> PIRLPNPMIGFGVPNEPGLITHRSLPELARGPPFFYYENVALTPKGVWETISRHLFEIPPEFVDSKYFCVAARKRGYIHNLPINNRFQIQPPPKYTIHDAFPLSKRWWPEWDKRTKLNCILTCTGSAQLTNRIRVALEPYNEEPEPPKHVQRYVIDQCKKWNLVWVGKNKAAPLEPDEMESILGFPKNHTRGGGMSRTERFKSLGNSFQVDTVAYHLSVLKPIFPHGINVLSLFTGIGGGEVALH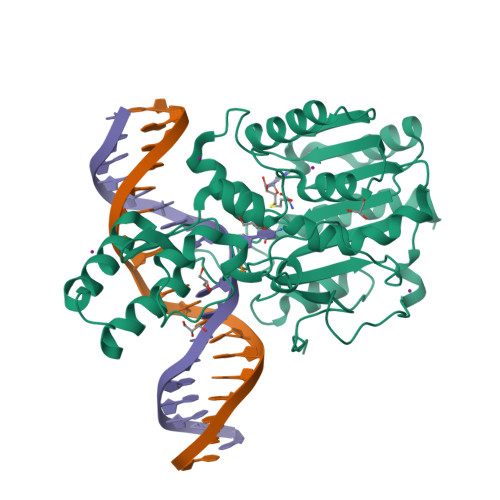RLQIKMKLVVSVEISKVNRNILKDFWEQTNQTGELIEFSDIQHLTNDTIEGLMEKYGGFDLVIGGSPCNNLAGGNRVSRVGLEGDQSSLFFEYCRILEVVRARMRGS>SSKSCLVARIQLLNNEFVEFTLSVESTGQESLEAVAQRLELREVTYFSLWYYNKQNQRRWVDLEKPLKKQLDKYALEPTVYFGVVFYVPSVSQLQQEITRYQYYLQLKKDILEGSIPCTLEQAIQLAGLAVQADFGDFDQYESQDFLQKFALFPVGWLQDEKVLEEATQKVALLHQKYRGLTAPDAEMLYMQEVERMDGYGEESYPAKDSQGSDISIGACLEGIFVKHKNGRHPVVFRWHDIANMSHNKSFFALELANKEETIQFQTEDMETAKYIWRLCVARHKFYRLNQCNLQTQTVTV[2x]

PTPN21 belongs to the four-point-one, ezrin, radixin, moesin (FERM) domain–containing protein tyrosine phosphatases (PTP) and plays important roles in cytoskeleton-associated cellular processes like cell adhesion, motility, and cargo transport. Because of the presence of a WPE loop instead of a WPD loop in the phosphatase domain, it is often considered to lack phosphatase activity. However, many of PTPN21’s biological functions require its catalytic activity. Combined with biochemical analysis, we have found that PTPN21 PTP is weakly active and is autoinhibited by association with its FERM domain.

The N terminus FERM domain of PTPN21 (18 to 319) crystallized in space group P212121 with two molecules in the asymmetric unit, and the structure was determined at 2.1 Å. The two molecules are quite similar and adopt the three-lobed cloverleaf architecture (F1, F2, and F3) characteristic of the archetypical FERM domains found in radixin, moesin, and focal adhesion kinase. The F1 lobe (21 to 106) exhibits a ubiquitin-like fold and is composed of a five-stranded β sheet covered by two α helices. The F2 lobe (107 to 216) contains a core four-helix bundle that resembles acyl-CoA binding protein. The F3 lobe (219 to 308) consists of an antiparallel seven-stranded β sandwich with a C-terminal α helix (α8) in between, similar to the pleckstrin homology superfold. The F2 and F3 lobes both interact with F1, and this arrangement holds the three subdomains together. Fortuitously, two MPD molecules were buried in the hydrophobic pockets of the F2 lobe. MPD binding caused the PTPN21 FERM Y158 region to adopt a different conformation. Using PIP-Strips lipid dot blot analysis, we found that PTPN21 FERM associated with certain phosphatidylinositol phosphate species as well as phosphatidic acid. Triple mutation of positively charged residues (K82, K86, and K291) greatly weakened the FERM-lipid interaction.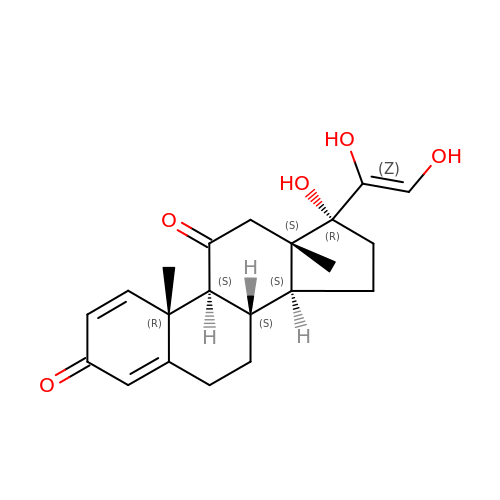17,21-DIHYDROXYPREGNA-1,4-DIENE-3,11,20-TRIONE | C21 H26 O5 | WZTZVUUYKIOIRV-LMZHSBCYSA-N The Munc13–1/α-RIM interaction is particularly interesting in this regard since its physiological importance has been demonstrated and both Munc13–1 and α-RIMs are involved in priming and plasticity. Our results suggest that a Munc13–1 homodimer–Munc13–1/α-RIM heterodimer switch regulates neurotransmitter release and some forms of presynaptic plasticity, and reveal the structural basis for homo- and heterodimerization. 2A domain can in fact establish two different types of interactions that lead to either homodimerization with itself or heterodimerization with the RIM2α ZF domain. Since the Munc13–1/α-RIM interaction competes with Munc13–1 homodimerization, this model predicts that Munc13–1 may exist in solution as a homodimer that needs to be disrupted in order to bind to α-RIMs at the active zone.

2A-domain homodimer at 1.44 Å resolution, designed a mutation that disrupts homodimerization, and solved the X-ray crystal structure at 1.78 Å resolution of a Munc13–1 fragment bearing this mutation bound to the RIM2α ZF domain. 2A domain of Munc13–1 encompasses approximately residues 3–130. 2A domain is sufficient and primarily responsible for homodimerization. 2A-domain crystals contains four monomers (referred to as monomers A–D). In contrast, homodimerization involves one side of the β-sandwich. This side contains the concave β-sheet, which interacts with the concave β-sheet of the other monomer in an antiparallel fashion. The interaction involves strand–strand hydrogen bonds through the “naked” edges of the β-sheets, leading to the formation of a β-barrel–like structure. The physiological role of Munc13–1 homodimerization is currently unclear, but it is plausible that it may play an inhibitory role by hindering α-RIM binding or it may help to stabilize Munc13–1 in the cytoplasm, before engaging in interactions at the active zone.

>[4x]GGVMSLLCVGVKKAKFDGAQEKFNTYVTLKVQNVKSTTIAVRGSQPSWEQDFMFEINRLDLGLTVEVWNKGLIWDTMVGTVWIPLRTIRQSNEEGPGEWLTLDSQAIMADSEICGTKDPTFHRILLDAHFE>[2x]SNAMEGNMLYHRYLKPNSEYYKKIEVRGKDNIYELNDIPDTYAVFLDNESVWKHYHVKGSTLPEQGWKIHVTSSLEDSKDVLDKVARLCIDKKIEFKHLKDKDSFMKMNSKNANRASSGKFITIYPTNNEVFVELLEMISLAIQDFKKGPYILNDKRWKNSNVFYRYGGFKGIFNEHGEHCIRDKEGNLIKDQRNPFYQVPDFVKDFDDYLNTINNSGELENKGESRLGKYKIETALSFSNAGGV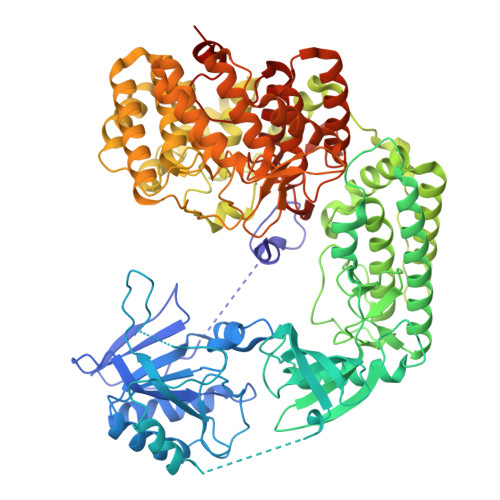YLATRKKDNLKVIIKEARPSAGLDGAAQDALARQKIEYDALKKLKDVSGVVNLIEYFQEWEHYFLVEEFIEGRDLRQWIAQEFPFFEDNNGMSNHIKDVKMILLQLLDLIDSMHNQGVAMGDLQPANIMVTEDLTVRIIDFETAMPVNSDDRPAMLTTGFVSHEMKVSGARDWFGFKRLVRYLALPVLTSEDLEGYLQYNHLNWIKENYGYEFYSFIVDLQEKCDKRIKDYQTFIPKEINLNDQTSDFNLTSIINKLIIGVESSLTNDERFINGDIRQFEMNGGKFNFLTGGSGAAFTLTKNKSSIAEVDKWIQSVLLDNLPLIEEDGLFTGKTGILALLYDKGYKEVVLNELKILKDNINQTDISIRSGLSGIGLFVISLYLETENKEYLKLAKDLERMIKLNRAKDKQLKVKDWMAVDIGVIDGLSGVSLFYSALYSVTQNQKYLEEAEVLIKEDLESTKKDDVTGVLQTVDNKNRLLPYLSGGSIGVAISIWFLNHVSGQDLYREEMNSILKLSKTRCTISGGLFDGAGSFLLIPSMVKNDKNREVILNEVLNLLNIFLIEKNSYYVYPGQFSYRLADDVYTGSSGIILALMGVIKGNPLYWLPLVNSDEFLARTKVKDLSVTSGKI(3~{S})-3-(cyclohexylmethyl)-6,8-bis(oxidanyl)-3,4-dihydroisochromen-1-one 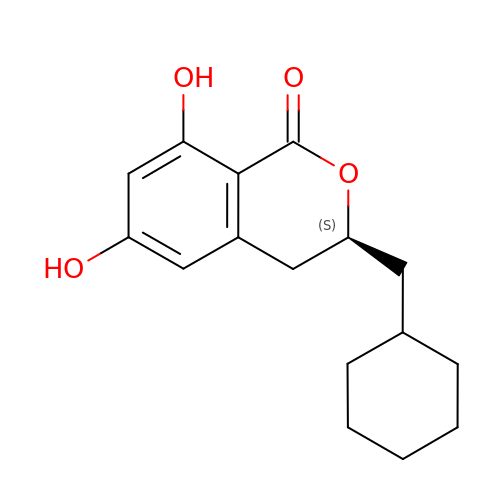| C16 H20 O4 | DGZHGFFAXFRYBW-ZDUSSCGKSA-N Amprolium | C14 H19 N4 | 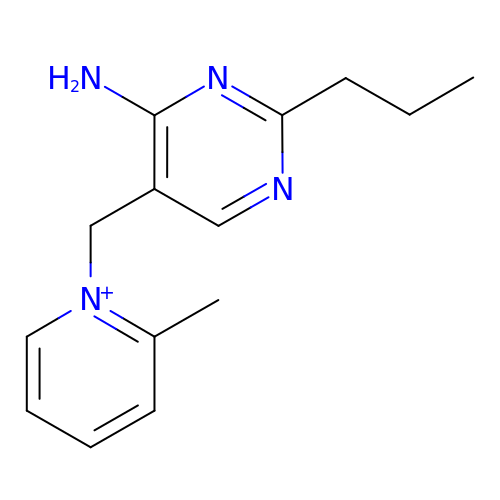IPZFPROOBOUEIG-UHFFFAOYSA-N5-{(3S)-1-[(Z)-iminomethyl]piperidin-3-yl}-2-(4-phenoxyphenoxy)pyridine-3-carboxamide 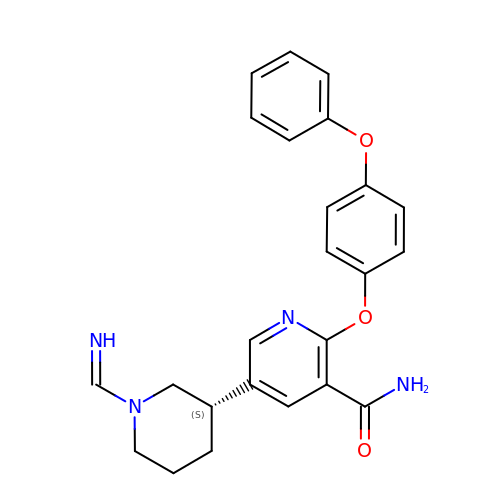| C24 H24 N4 O3 | CLMOAHOTUBCRAU-GGMUZDTOSA-N>[12x]GAMGIGKSPTGIQGFDELTLGGLPTGRPSLVCGSAGCGKTLFASTFLINGVRDHGEPGVFVTFEERPEDIVNNVASLGFELDKLIEEEKIAIEHIAVDPSEVAEIGDYDLEGLFLRLELAIDTVGAKRVVLDTIESLFSAFSNPAILRAEIRRLFDWLKERGLTTVITAERGDGALTRQGLEEYVSDCVILLDHRVENQISTRRLRIVKYRGTAHGTNEYPFLIDTDGFSVLPVSALGLLHQVHEERIASGVPDLDAMMAGGGFFRGSSILVSGVAGAGKSSLAAHFAAAACARGERAMYFSFEEAADQAVRNMRSLGLDLGRWRDAGLLRFMATRPTFYSLEMHLAVILREVMRFEPSVVVLDPISAFTESGDRLEVQSMLLRIVDFLKNRGITGIFTHLAHSQNEATTDAGLSSLMDGWVLMLNREVNGEFNRELYLLKARGMAHSNQVREFLMSDRGISLLPPHLGEGGALTGTARKAEEARLRRAEIERQTELGRLQQQIEQRRRRARAQIEALEAELQAEEIALKALVESESAHERQRLADADTLARSRGNERFADLLMNKGE

Here we investigate the primordial circadian clock in Rhodobacter sphaeroides, which contains only KaiBC, to elucidate its inner workings despite missing KaiA. Using a combination of X-ray crystallography and cryogenic electron microscopy, we find a new dodecameric fold for KaiC, in which two hexamers are held together by a coiled-coil bundle of 12 helices. This interaction is formed by the carboxy-terminal extension of KaiC and serves as an ancient regulatory moiety that is later superseded by KaiA. Our kinetic data identify the difference in the ATP-to-ADP ratio between day and night as the environmental cue that drives the clock.

A closer inspection of the CII domains in KaiCRS and KaiCSE/TE (Thermosynechococcus elongatus BP-1 referred to as KaiCTE) showed an obvious difference in A loop orientations: an extended conformation in KaiCRS compared with a buried orientation in KaiCSE/TE. Furthermore, the sequence similarity between KaiCRS and KaiCSE is less than 30% for the A loop and residues considered important for stabilization of this loop in its buried orientation (that is, the 422 loop and residues 438–444). Together, our structural and kinetic data support the idea that an exposed A loop is key for the KaiA-independent enhancement of nucleotide exchange and hence autophosphorylation in KaiCRS and perhaps other KaiBC-based systems. The dodecameric KaiCRS showed constitutive kinase activity owing to its extended C-terminal tail that forms a coiled-coil bundle with the opposing hexamer. This structure elicits a conformation akin to the exposed A loop conformation in KaiACSE, and autophosphorylation occurs within half an hour. Notably, the coiled-coil bundle provides additional hexameric stability. In detail, the KaiCRS dodecamer is stable for extended periods of time in the presence of only ADP, whereas for KaiCSE, oligomers are not observed under these conditions. Furthermore, the C-terminal residues of KaiCRS-S413E/S414E interacted with the CII domain of the opposite hexamer, whereas the lack of electron density for the last 30 residues in the wild-type structure indicates more flexibility in the dephosphorylated state. The wild-type protein dephosphorylated comparatively quickly (observed rate constant = 11.5 ± 0.8 h−1) in the presence of only ADP. Consistent with this accelerated dephosphorylation rate mediated by the coiled-coil domain, our crystallographic data showed a phosphate group on Ser414 for KaiCRS-Δcoil but not for the wild-type protein.>[2x]SLRSDLINALYDENQKYDVCGIISAEGKIYPLGSDTKVLSTIFELFSRPIINKIAEKHGYIVEEPKQQNHYPDFTL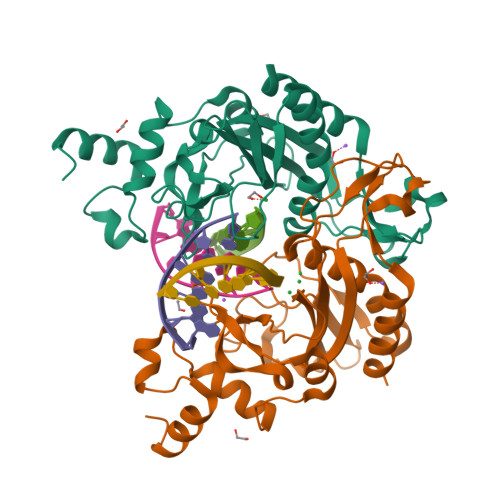YKPSEPNKKIAIDIKTTYTNKENEKIKFTLGGYTSFIRNNTKNIVYPFDQYIAHWIIGYVYTRVATRKSSLKTYNINELNEIPKPYKGVKVFLQDKWVIAGDLAGSGNTTNIGSIHAHYKDFVEGKGIFDSEDEFLDYWRNYERTSQLRNDKYNNISEYRNWIYRGRK4-CHLORO-BENZOIC ACID | C7 H5 Cl O2 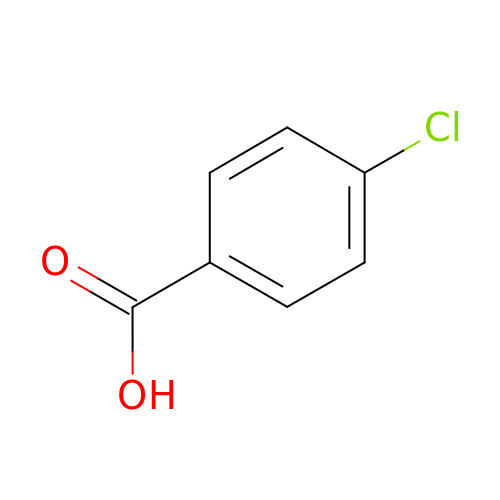| XRHGYUZYPHTUJZ-UHFFFAOYSA-N> GADDDKPIQVTQMPQL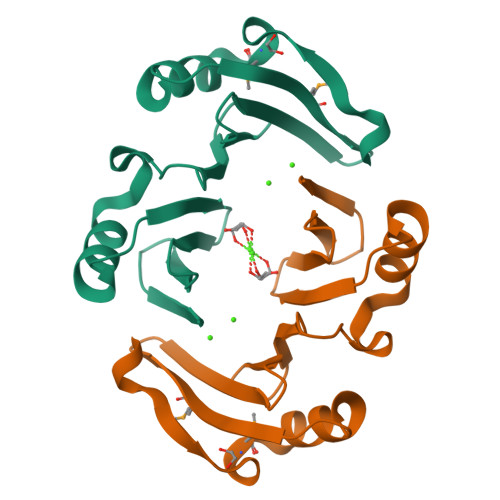AQQFIKQHFSDSKVALAKMESDFLYKSYEVIFTNGNKVEFDKKGNWEEVDCKHTSVPVAIIPAAIQKYVTTNYPDAKVLKIERDKKDYEVKLSNRTELKFDLKFNLIDIDN>[2x]GNMPVRYFIMKSSNLRNLEISQQKGIWSTTPSNERKLNRAFWESSIVYLVFSVQGSGHFQGFSRMSSEIGREKSQDWGSAGLGGVFKVEWIRKESLPFQFAHHLL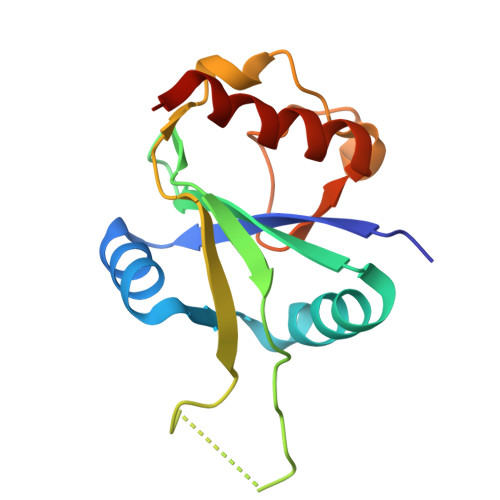NPWNDNKKVQISRDGQELEPLVGEQLLQLWERLPLG> KETAAAKMERQHLDS;> NYCNQMMKSRNLTKD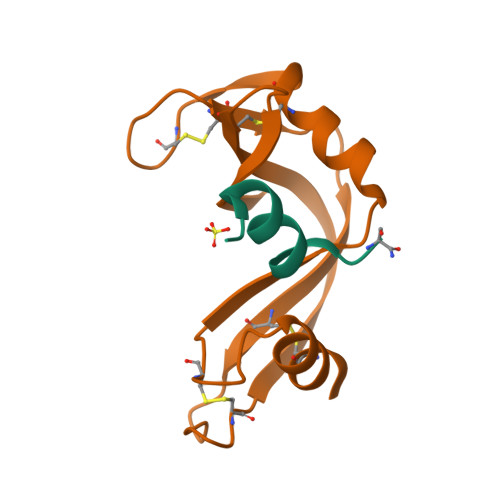RCKPVNTFVHESLADVQAVCSQKNVACKNGQTNCYQSYSTMSITDCRETGSSKYPNCAYKTTQANKHIIVACEGNPYVPVHFDASV Rai1 homologs share several highly conserved sequence motifs, and our structural studies show that they are located in the active site region, mediating the binding of the divalent metal ions and/or the RNA. We have found substantial variations in the activity profiles of the Rai1 homologs, and discovered that some of them possess a new 5′ triphosphonucleotide hydrolase (TPH) activity. The overall structures of CaRai1, AgRai1 and SsRai1 are similar to those of SpRai1 (16), KlDxo1 (18), and MmDXO. Each structure contains two mixed β-sheets that are surrounded by α-helices.

The rms distance is 0.62 Å for AgRai1, and small changes for helix αF (containing motif V) and other regions are visible, although these changes are unlikely to seriously affect RNA binding. The structures of the AgRai1 and CaRai1 free enzymes will not be described further here. AgRai1 has the strongest decapping and exonuclease activities in our assays. The αC helix is absent in AgRai1 but contains more than four turns in CaRai1 and SsRai1, which also have a longer αD helix. The results also consistently show that AgRai1 has the strongest activities in the buffer conditions tested.

> MVFESELLLQRRLATTALKQPKELGYYSTNVGGELKVMDESNLSYYYLPDADIEKHIDLSAGARKFQDEQAEAEDDTGSLHGLLQTLMEYERRKSKKVNADIIAFRGQVKRLIHCAFGGHATDVDMYVMSFDGQLFIRAARKKLEFPTSPRESWAYLAYYSGYKFERMALLDRPVAETPREVLESRGKQVVRNGPQYKTVVRTGVGEHKLVLGAEVDGIFDFREPTGDNLKHYVELKVAKKVQTLKDATNFEQKLFSVWLQCFLVGINRVIIGFRDEKFVLKSVEEFSTSEIPLLLKSTGLRNACVDAIKWYGALTKWLCELPRGPEDDFKLYRLSCSRGALHLRQLHDEDLANGDDIIPGWFREWRRSLSKSHGS methyl 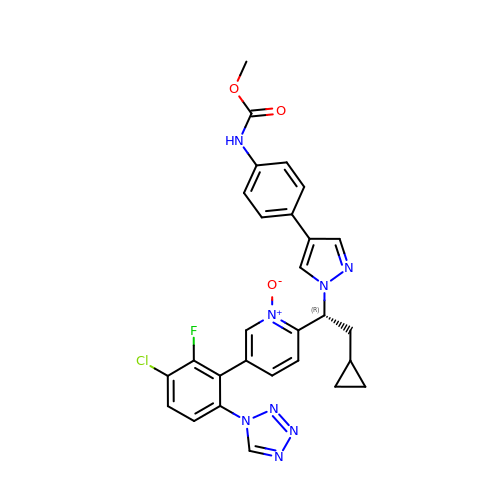~{N}-[4-[1-[(1~{R})-1-[5-[3-chloranyl-2-fluoranyl-6-(1,2,3,4-tetrazol-1-yl)phenyl]-1-oxidanyl-pyridin-2-yl]-2-cyclopropyl-ethyl]pyrazol-4-yl]phenyl]carbamate | C28 H24 Cl F N8 O3 | UEZIPJPABXSKCS-RUZDIDTESA-N>MTSAEMTSPNNNSEHQAIAKMRTMIEGFDDISHGGLPIGRSTLVSGTSGTGKTLFSIQFLYNGIIEFDE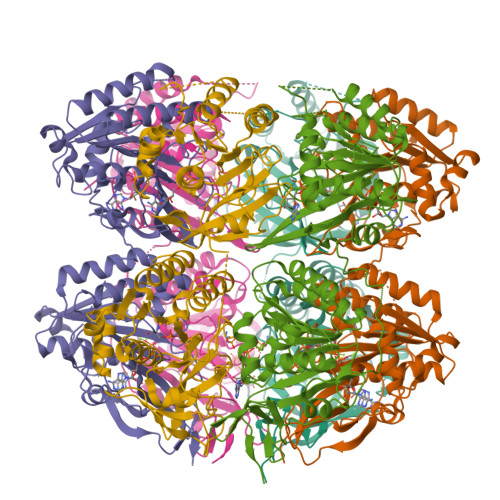PGVFVTFEETPQDIIKNARSFGWDLAKLVDEGKLFILDASPDPEGQEVVGGFDLSALIERINYAIQKYRARRVSIDSVTSVFQQYDASSVVRRELFRLVARLKQIGATTVMTTERIEEYGPIARYGVEEFVSDNVVILRNVLEGERRRRTLEILKLRGTSHMKGEYPFTITDHGINIFPLGAMRLTQRSSNVRVSSGVVRLDEMCGGGFFKDSIILATGATGTGKTLLVSRFVENACANKERAILFAYEESRAQLLRNAYSWGMDFEEMERQNLLKIVCAYPESAGLEDHLQIIKSEINDFKPARIAIDSLSALARGVSNNAFRQFVIGVTGYAKQEEITGLFTNTSDQFMGAHSITDSHISTITDTIILLQYVEIRGEMSRAINVFKMRGSWHDKAIREFMISDKGPDIKDSFRNFERIISGSPTRITVDEKSELSRIVRGVQEKGPES[12x]(E)-2-(4-carbamimidoylbenzylideneaminooxy)-2-methylpropanoic acid | C12 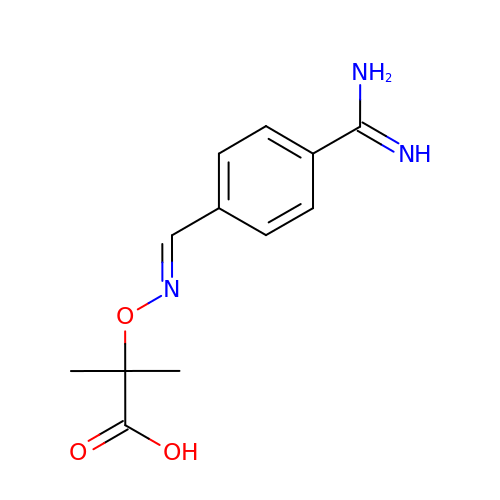H15 N3 O3 | XNCYVTKDNMFVND-VIZOYTHASA-N>GSSGSSGPSSPSIDQVEPYSSTAQVQFDEPEATGGVPILKYKAEWRAVGEEVWHSKWYDAKEASMEGIVTIVGLKPETTYAVRLAALNGKG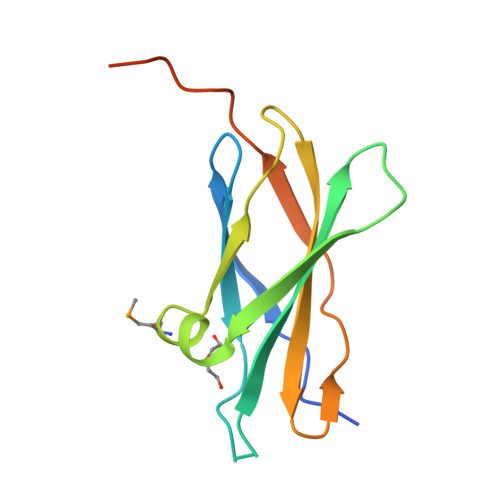LGEISAASEFKTQPVREPSAPKLEGSGPSSG[3x]> HHHHMPVFHTRTIESILEPVAQQISHLVIMHEEGEVDGKAIPDLTAPVAAVQAAVSNLVRVGKETVQTTEDQILKRDMPPAFIKVENACTKLVQAAQMLQSDPYSVPARDYLIDGSRGILSGTSDLLLTFDEAEVRKIIRVCKGILEYLTVAEVVETMEDLVTYTKNLGPGMTKMAKMIDERQQELTHQEHRVMLVNSMNTVKELLPVLISAMKIFVTTKNSKNQGIEEALKNRNFTVEKMSAEINE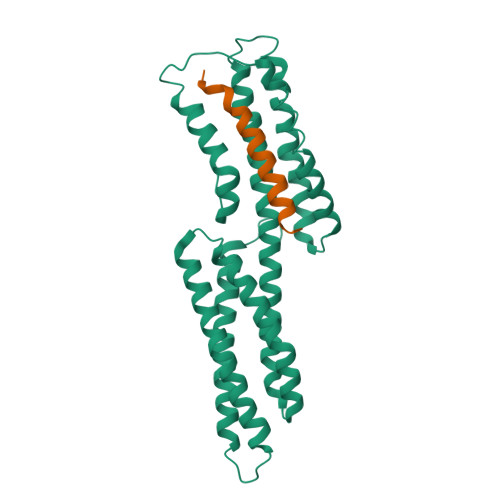IIRVLQLTSWDEDAW;> YTKKELIESARKVSEKVSHVLAALQA> MIIPALDLIGGTVVRLHQGDYARQRDYGNDPLPRLQDYAAQGAGVLHLVDLTGAKDPAKRQIPLIKTLVAGVNVPVQVGGGVRTEEDVAALLK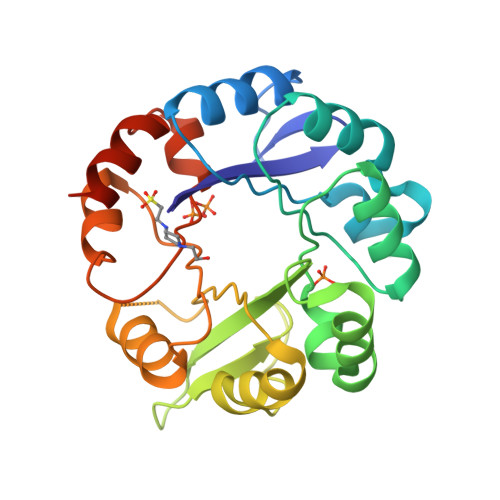AGVARVVIGSTAVKSPDVVKGWFERFGAQALVLALDVRIDEHGTKQVAVSGWQENSGVSLEQLVETYLPVGLKHVLCTDISRDGTLAGSNVSLYEEVCARYPQIAFQSSGGIGDIDDIAALRGTGVRGVIVGRALLEGKFTVKEAIQCWQNVKGHHHHHH>[2x]GGSGAKLLQILNVRVVGSGERVVVLSHGFGTDQSAWSRVLPYLTRDHRVVLYDLVCAGSVNPDHFDFRRYDNLDAYVDDLLAILDALRIPRCAFVGHSVSAMIGILASIRRPDLFAK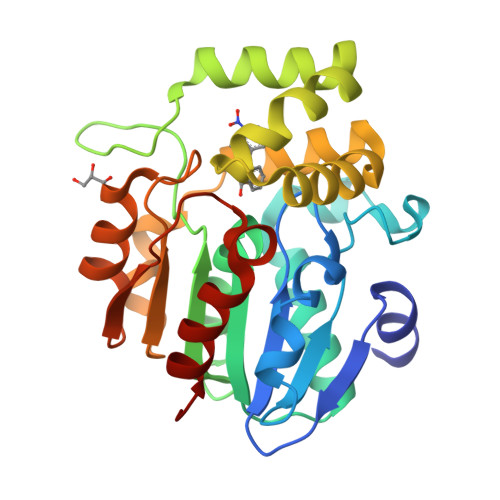LVLIGASPRFLNDSDYHGGFELEEIQQVFDAMGANYSAWATGYAPLAVGADVPAAVQEFSRTLFNMRPDISLHVCQTVFKTDLRGVLGMVRAPCVVVQTTRDVSVPASVAAYLKAHLGGRTTVEFLQTEGHLPHLSAPSLLAQVLRRALARY> MTDTTNSIKHVISPLARQTLQDRDLTRPVAGKRPIRLLPWLQVVKIGGRVMDRGADAILPLVEELRKLLPEHRLLILTGAGVRARHVFSVGLDLGLPVGSLAPLAASEAGQNGHILAAMLASEGVSYVEHPTVADQLAIHLSATRAVVGSAFPPYHHHEFPGSRIPPHRADTGAFLLADAFGAAGLTIVENVDGIYTADPNGPDRGQARFLPETSATDLAKSEGPLPVDRALLDVMATARHIERVQVVNGLVPGRLTAALRGEHV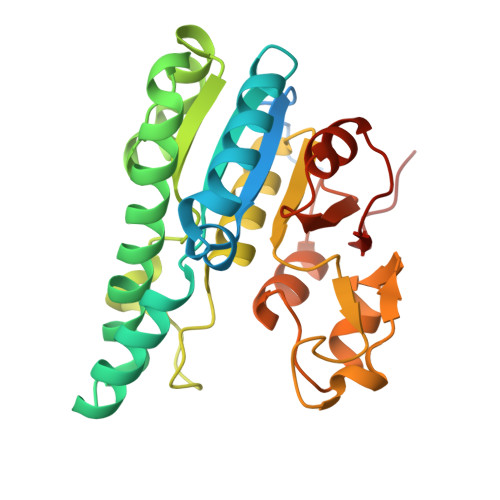GTLIRTGVRPA Human noroviruses (HuNoVs) cause sporadic and epidemic viral gastroenteritis worldwide. ORF2 encodes the major capsid protein VP1 that encapsidates the (+) sense ssRNA genome and ORF3 codes for the minor structural protein VP2 that is suggested to be located internally in the capsid. All these structures showed that the capsid exhibits T = 3 icosahedral symmetry, with a diameter of ~400 Å, composed of 90 dimers of the capsid protein VP1 that consists of an internal N-terminal arm (NTA) and two distinct domains separated by a flexible hinge. In the capsid architecture, the N-terminal domain ‘ties’ the VP1 subunits through a network of interactions facing the interior of the capsid, the S domain forms the icosahedral shell, and the P domain protrudes from the S domain.

The final resolution of the cryo-EM structure is ~3.8 Å as estimated by Fourier Shell Correlation (FSC) of 0.143. The quality of the 3.8 Å cryo-EM map allowed the unambiguous fitting of all the three quasi-equivalent VP1 subunits in the T = 3 icosahedral capsid, which showed well-defined densities for their S and P domains. In all the three quasi-equivalent subunits, the P domain rests on the S domain in the resting conformation, as observed in the crystal structure. This is also evident in the cut-away view of the cryo-EM map, which shows continuous density between the S domain and the P domain. The conformations of the A and B subunits are the same as in the X-ray structure, whereas the C subunit is ‘locked’ into a singular conformation selected from one of the 15 conformations observed in the crystal structure to adhere to the icosahedrally symmetric organization. In both the crystal and solution, the capsid protein VP1 assumes a resting state stabilized by an elaborate network of NTA linking the capsid subunits and the interactions between the S and P domains, as expected in a T = 3 icosahedral capsid. A novel finding is the metal ion binding at the dimeric interface of the P domain that further stabilizes the resting conformation. Although the metal ion observed in our crystal structure is likely Cd2+, based on the composition of the crystallization buffer, the nature of the metal ion in the cryo-EM density is uncertain.

>MKMASSDASPSDGSTANLVPEVNNEVMALEPVVGAAIAAPVAGQQNVIDPWIRNNFVQAPGGEFTVSPRNAPGEILWSAPLGPDLNPYLSHLARMYNGYAGGFEVQVILAGNAFTAGKIIFAAVPPNFPTEGLSPSQVTMFPHIIVDVRQLEPVLIPLPDVRNNFYHYNQSNDPTIKLIAMLYTPLRANNAGDDVFTVSCRVLTRPSPDFDFIFLVPPTVESRTKPFTVPILTVEEMTNSRFPIPLEKLFTGPSGAFVVQPQNGRCTTDGVLLGTTQLSPVNICTFRGDVTHIAGTHDYTMNLASQNWNNYDPTEEIPAPLGTPDFVGKIQGVLTQTTRGDGSTRGHKATVSTGSVHFTPKLGSVQFTTDTNNDLETGQNTKFTPVGVVQDGNSAHQNEPQQWVLPNYSGRTGHNVHLAPAVAPTFPGEQLLFFRSTMPGCSGYPNMNLDCLLPQEWVLHFYQEAAPAQSDVALLRFVNPDTGRVLFECKLHKSGYVTVAHTGPHDLVIPPNGYFRFDSWVNQFYTLAPMGNGAGRRRAL[3x]>M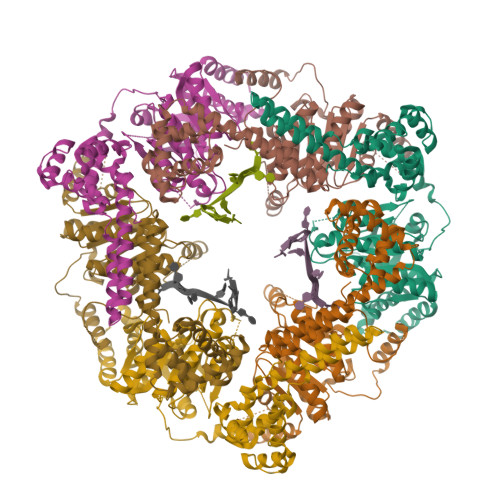SELFSERIPPQSIEAEQAVLGAVFLDPTALTLASERLIPEDFYRAAHQKIFHAMLRVADKGEPVDLVTVTAELAALEQLEEVGGVSYLSELADSVPTAANVEYYARIVEEKSLLRRLIRTATSIAQDGYTREDEIDVLLDEAERKIMEVSQRKHSGAFKNIKDVLVQTYDNIEMLHNRNGDITGIPTGFTELDRMTSGFQRSDLIIVAARPSVGKTAFALNIAQNVATKTNENVAIFSLEMSAQQLVMRMLCAEGNINAQNLRTGKLTPEDWGKLTMAMGSLSNAGIYIDDTPSIRVSDIRAKCRRLKQESGLGMVVIDYLQLIQGSGRNRENRQQEVSEISRSLKALARELEVPVIALSQLSRSVEQRQDKRPMMSDLRESGSIEQDADIVAFLYRDDYYNKDSENKNIIEIIIAKQRNGPVGTVQLAFIKEYNKFVNLERRFDEAQIPPGA[2x]>[3x]GPGSLSQASADLEATLRHKLTVMYSQINGASRALDDVRNRQQDVRMTANRKVEQLQQEYTEMKALLDASETTSTRKIKEEEKRVNSKFDTIYQILLKKKSEIQTLKEEIEQSLTKRDEFEFLEKASKLRGISTKPVYIPEVELNHKLIKGIHQSTIDLKNELKQCIGRLQELTPSSGDPGEHDPASTHKSTRP;>[3x]GPGTMASVPASRYLTDMTLEEMSREWSMLIPKQKVAGPLCIRMDQAIMDKNIILKANFSVIFDRLETLILLRAFTEEGAIVGEISPLPSLPGHTAEDVKNAVGVLIGGLEWNDNTVRVSETLQRFAWRSSNENGRPPLTPKQKREMAGTIRSEV

Tripartite motif (TRIM) family proteins are RING-type E3 ligases that play key regulatory roles in innate immune signalling pathways that lead to the induction of a type I interferon (IFN) response and production of inflammatory cytokines through activation of the IRF3 and NF-κB transcription factors. Activation of RIG-I initiates a signalling cascade that depends on the E3 ligase activity of TRIM25 and induces the production of IFNs and inflammatory cytokines. An example is non-structural protein 1 (NS1) of influenza A viruses (IAV), a multifunctional virulence factor that binds many host proteins during infection, including TRIM2527–29. To understand NS1-mediated inhibition of TRIM25 activity on a molecular level we have determined crystal structures of the CC domain of TRIM25 in complex with NS1-FL and the isolated ED, and of a TRIM25 CC-PRYSPRY fragment, which includes the RIG-I-recognition domain of TRIM25.

To gain molecular insight into the interaction between NS1 and TRIM25 we determined the crystal structure of the NS1-ED/TRIM25-CC complex at 2.8 Å resolution by molecular replacement (R/Rfree = 0.20/0.22). The complex crystallised in space group C222 with three copies of each NS1-ED and TRIM25-CC monomer in the asymmetric unit. Symmetry analysis shows that each NS1-ED binds to a TRIM25-CC dimer via two separate interfaces, interface A and interface B, which bury 872 and 611 Å2, respectively, of solvent accessible surface. The biggest difference between apo TRIM25-CC and the NS1-bound state is seen in the linker connecting helix α2 to the central helix α3, which is pushed from its position in the apo TRIM25-CC structure towards helix α1 due to contacts by NS1-ED from interface A. This copy of NS1-ED makes contacts with both TRIM25 chains within the CC dimer via a highly conserved motif of NS1 that includes a short α helix comprising residues 95–99. Previous mutational analysis identified E96 and E97 in this motif as crucial for TRIM25 binding and inhibition of interferon production. Our structure now shows that the side chains of E96 and E97 point away from the binding interface with TRIM25. However, they form a network of contacts within NS1-ED, especially between the side chains of E96 and R100, which is likely important to maintain the structural integrity of this helix. Instead, L95ED of this helix is a key element of the interface and contacts a hydrophobic pocket of TRIM25 formed by residues from both chains of the CC including V223CC, F274CC, I277CC, I324CC and V327CC. This interaction is further stabilised by a hydrogen bond between the backbone of L95ED and the side chain of E326CC. Interface B involves loop-forming NS1-ED residues 139-143 that contact the central four-helical bundle of TRIM25-CC with R140ED at its centre.>[2x]MGSSYHHHHHHSSGENLYFQHMKHGRVFIIKSYSEDDIHRSIKYNIWCSTEHGNKRLDAAYRSMNGKGPVYLLFSVNGSGHFCGVAEMKSAVDYNTCAGVWSQDKWKGRFDVRWIFVKDVPNSQLRHIRLENNENKPVTNSRDTQEVPLEKAKQVLKIIASYKHTTS

The YTH (YT521-B homology) domain-containing proteins are a family of RNA-binding proteins that specifically recognize N 6-methyladenosine (m6A), the most abundant internal modification in eukaryotic RNA. In contrast, the DF proteins (DF1, DF2, and DF3) are mainly cytoplasmic and play essential roles in mRNA translation, stability, and degradation. Our study focuses on DF2, which is involved in multiple types of cancer, including prostate cancer, MYC-driven breast cancer, and acute myeloid leukemia (AML). We have also presented the crystal structures of DF2 in complex with six ligands, which represent six distinct chemotypes (compounds 3–6, 13, and 15).

Other molecules closely related to the thiobarbiturates were identified as interesting binders: barbiturates 11 and 12, triazine 13, and condensed bicycles 14–16. The X-ray crystal structures of compounds 13 and 15 confirm their binding, again showing the sulfur atom interacting within the lipophilic tryptophan cage. Compound 15 can establish all of the interactions previously discussed: in addition to the interactions of m6-adenine, it can interact with both D422 and D528. Unfortunately, the multiple interactions of compound 15 do not translate into a very strong binding (IC50 = 86 μM). Moreover, in the present campaign the crystal structure of DF2 in the complex with compound 15 guided the derivatization of compound 14, which has a similar scaffold and binding mode. We were not able to determine the crystal structure of 14 in complex with DF2. Thus we hypothesized a similar binding mode as in the crystal structure with compound 15. Figure A shows the two reference poses obtained for compound 14 compared to the crystal structure of compound 15. In pose A, the carbonyl oxygen interacts with the backbone NH of Y418, as observed for the crystal structure with compound 15.>GGYVLGS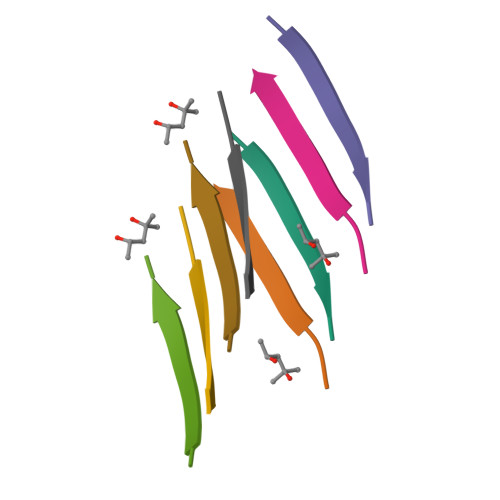[2x]> PMTLGYWNIRGLAHSIRLLLEYTDSSYEEKKYTMGDAPDYDRSQWLNEKFKLGLDFPNLPYLIDGTHKITQSNAILRYIARKHNLCGESEKEQIREDILENQFMDSRMQLAKLCYDPDFEKLKPEYLQALPEML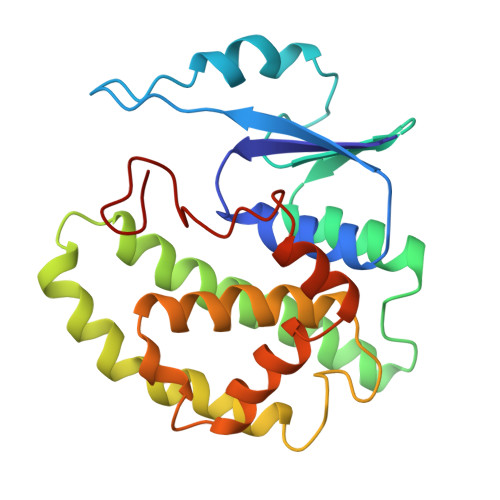KLYSQFLGKQPWFLGDKITFVDFIAYDVLERNQVFEPSCLDAFPNLKDFISRFEGLEKISAYMKSSRFLPRPVFTKMAVWGNK>GSMSEQSICQARAAVMVYDDANKKWVPAGGSTGFSRVHIYHHTGNNTFRVVGRKIQDHQVVINC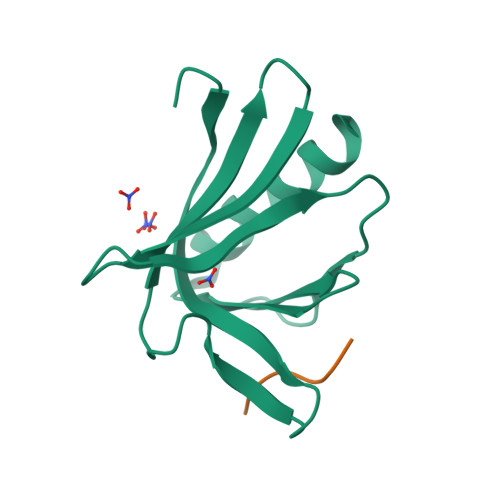AIPKGLKYNQATQTFHQWRDARQVYGLNFGSKEDANVFASAMMHALEVL[2x]> SYV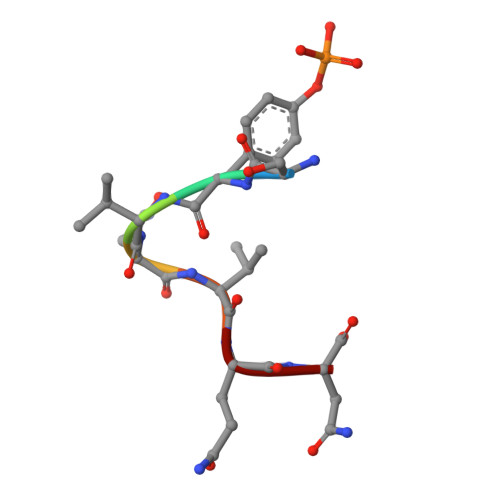NVQN>MSLITMKKIGVILSGCGVYDGSEIHEAVLTLLAISRSGAQAVCFAPDKQQVDVINHLTGEAMTETRNVLIEAARITRGEIRPLAQADAAELDALIVPGGFGAAKNLSNFASLGSECTVDRELKALAQAMHQAGKPLGFMCIAPAMLPKIFDFPLRLTIGTDIDTAEVLEEMGAEHVPCPVDDIVVDEDNKIVTTPAYMLAQNIAEAASGIDKLVSRVLVL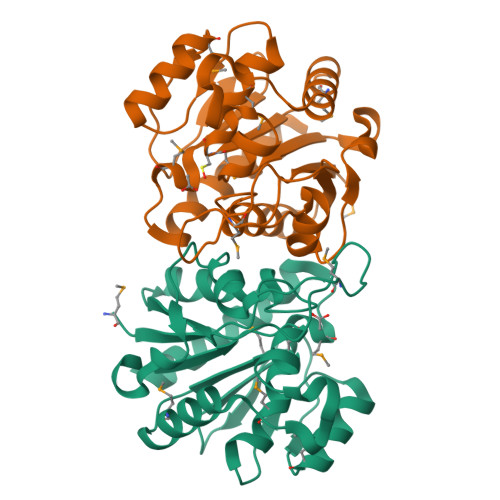AEEGGSHHHHHH[2x]The starting point of the engineering efforts reported here is a Kemp eliminase we previously obtained through minimalist design on a β-lactamase background. Our design took advantage of the conformational flexibility of an ancestral β-lactamase scaffold to produce both a suitable cavity and a catalytic base within it through a single mutation, while a second mutation enhanced relevant interactions at the de novo active site. Kemp elimination is a straightforward proton–abstraction reaction that can be performed by a simple molecular machinery consisting, at the bare minimum, of a catalytic base. FuncLib does not per se predict mutations that enhance catalysis, but rather suggests variants with multiple mutations that generate stabilizing interacting networks at the active site, thus focusing the search to safe regions of the sequence space.

Finally, we have used X-ray crystallography to determine the 3D-structures of the catalytically optimized GNCA4-2, GNCA4-12 and GNCA4-19 variants, the first of which has a transition state analogue bound at the de novo active site. These particular structures were chosen as they are all highly active variants, in terms of the measured rates within the available substrate concentration range, with improved catalytic parameters over GNCA4-WT. The protein backbones of these new structures are essentially superimposable with that of the background GNCA4-WT variant and, therefore, the observed enhancement of catalysis is likely linked to small rearrangements in the de novo active site. To assess this, we also performed EVB simulations on the variants for which crystal structures were available: GNCA-2, GNCA-12 and GNCA-19. For these variants, the calculated values fall to within 1.3 kcal mol–1 of the experimental values, and can deviate by up to 2.2 kcal mol–1 from the values calculated from the FuncLib predicted structures. In the case of GNCA-2, which has the largest deviation between the calculated activation free energies using the crystal and FuncLib structures (ΔΔG‡calc = 2.2 kcal mol–1 with the crystal structure giving better agreement with experiment), we observed subtle structural differences the crystal and FuncLib structures (Fig. S10†). Specifically, we observe different rotamers of the R256 and L291 side chains, as well as also subtle displacements of both the side chain of the catalytic base D229 (which is further from the substrate in the FuncLib predicted structure). The shift in the position of the catalytic base D229 in particular likely plays a significant role in the higher calculated activation free energy for this variant when using the FuncLib predicted structure as a starting point. We note that we have attempted to further refine our EVB calculations by exploring other approaches to generate the starting structures, such as predicting mutations using SCWRL63 or inserting point mutations manually using the Dunbrack rotamer library, as implemented in Chimera.

>MAAALSEQLAELEKRSGGRLGVAVLDTATGRRFGYRGDERFPMCSTFKALLAAAVLARVDQGKENLDRRITYGKEDLVDYSPVTEKHVGDGMTVAELCEAAITYSDNTAANLLLEALGGPAALTAFLRSIGDNVTRLDRWEPELNTAAPGDPRDTTTPAAMAATLRTLLLGDVLSPASRQQLVDWLIANKTGDKRLRAGLPADDRVGDKTGTGEHGTTNDIAVVWPPNRAPIFLAVYLTESQVDADARDAVIAEVARLVVAAWLHHHHH[3x]> XA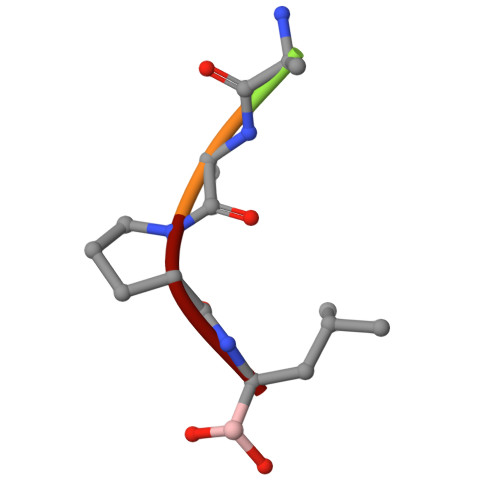APL> EFMVSLPRMVYPQPKVLTPCRKDVLVVTPWLAPIVWEGTFNIDILNEQFRLQNTTIGLTVFAIKKYVAFLKLFLETAEKHFMVG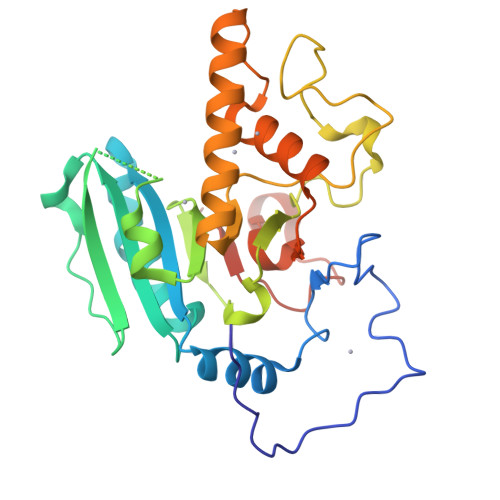HRVHYYVFTDQPAAVPRVTLGTGRQLSVLEVGAYKRWQDVSMRRMEMISDFCERRFLSEVDYLVCVDVDMEFRDHVGVEILTPLFGTLHPSFYGSSREAFTYERRPQSQAYIPKDEGDFYYMGAFFGGSVQEVQRLTRACHQAMMVDQANGIEAVWHDQSHLNKYLLRHKPTKVLSPEYLWDQQLLGWPAVLRKLRFTAVPKNHQAVRNPE> GPMTLYSKKDIVQQARNLAKMISETEEVDFFKRAEAQINENDKVSTIVN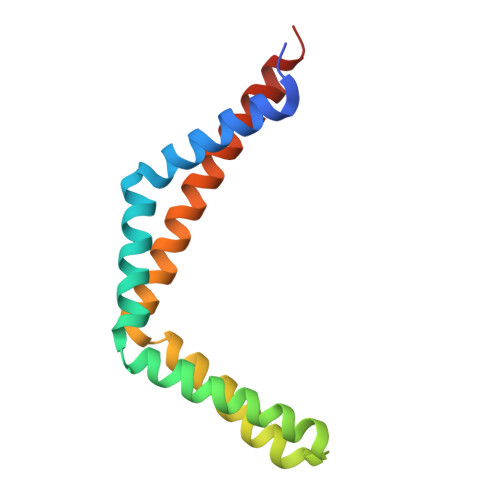QIKALQKQAVNLKHYEKHEALKQVEAKIDALQEELEEIPVIQEFRDSQMEVNDLLQLVAHTISNQVTNEIITSTG>MHHHHHHHHMDSRSPSLPDDRPDPPEQHLDARAGATLRGTAGPRGVRRILPFLRPAVIASIAYMDPGNFATNIEGGARYGYSLLWVILAANLMAMVIQNLSANLGIASGRNLPELIRERWPRPLVWFYWIQAELVAMATDLAEFLGAALAIQLLTGLPMFWGAVVTGVVTFWLLNLQKRGTRPLELAVGAFVLMIGVAYLVQVVLARPDLAAVGAGFVPRLQGPGSAYLAVGIIGATVMPHVIYLHSALTQGRIQTDTTEEKRRLVRLNRVDVIAAMGLAGLINMSMLAVAAATFHGKNVENAGDLTTAYQTLTPLLGPAASVLFAVALLASGLSSSAVGTMAGDVIMQGFMGFHIPLWLRRLITMLPAFIVILLGMDPSSVLILSQVILCFGVPFALVPLLLFTARRDVMGALVTRRSFTVIGWVIAVIIIALNGYLLWELLGG[2x]

Natural resistance-associated macrophage proteins (Nramps) are APC-superfamily transition metal transporters that enable uptake of rare micronutrients such as Mn2+ in plants and bacteria and Fe2+ in animals. Nramps bind and/or transport biologically-essential divalent metals such as Mn2+, Fe2+, Co2+, Ni2+, Cu2+, Zn2+—and toxic metals like Cd2+, Pb2+, and Hg2+—but not the abundant alkaline earth metals Mg2+ and Ca2+. Metal uptake by Nramps is typically stimulated by acidic pH and accompanied by proton influx. Nramps have 11 or 12 TMs, the first ten forming a LeuT fold, as seen in structures of three bacterial Nramp homologs, including our model system Deinococcus radiodurans (Dra)Nramp.

Adding steric bulk along TM1a—for example a G45R mutation, which mimics a human anemia-causing mutation of a conserved glycine —prevented the opening of the extracellular vestibule and eliminated metal transport, emphasizing the importance of the alternating-access mechanism to DraNramp function. WT-like DraNramp (with the indicated reporter cysteine and a C382S mutation to remove the lone endogenous cysteine) maintains a dynamic conformational equilibrium—even in the absence of added metal substrate—such that either reporter can be fully modified by the thiol-specific N-ethylmaleimide (NEM) at high concentrations. G45R slightly increased A53C accessibility but fully protected A61C, indicating an outward-closed state that we will refer to as inward-locked based on these data and the structure described below. We have thus identified two complementary constructs that trap DraNramp in outward-locked (G223W) and inward-locked (G45R) states. Using lipidic cubic phase (LCP) to mimic the hydrophobic membrane environment, we crystallized and determined the structures of G45R and G223W to resolutions of 3.0 and 2.4 Å, respectively, both significantly improved from our earlier DraNramp structure (3.94 Å) (Table 1 and Figure 2—figure supplements 1–2). Unexpectedly, the G45R structure is not in an inward-open conformation with our Fab-bound Patch mutant but instead adopts an inward-occluded, metal-free state that may represent an intermediate conformation between inward-open and outward-open states in the DraNramp transport cycle. The major exception is TM1a, which swings ~45° to partially seal the inward aqueous cavity in the G45R structure, a motion we previously showed to be essential to the transport cycle. The intracellular ends of TM4 and TM5 also move slightly compared to their position in the inward-open state, further sealing the metal-binding site from the cytosol. Comparisons of the G45R and G223W structures indicate that, rather than preventing inward motion of TM1a as we had hypothesized, the G45R mutation precludes TM4-TM5 from fully closing the inner gate, as any bulkier replacement for that absolutely-conserved glycine in our outward-open G223W structure would clash with E176 on TM5.>SKIVKIIGREIIDSRGNPTVEAEVHLEGGFVGMAAAPSGASTGSREALELRDGDKSRFLGKGVTKAVAAVNGPIAQALIGKDAKD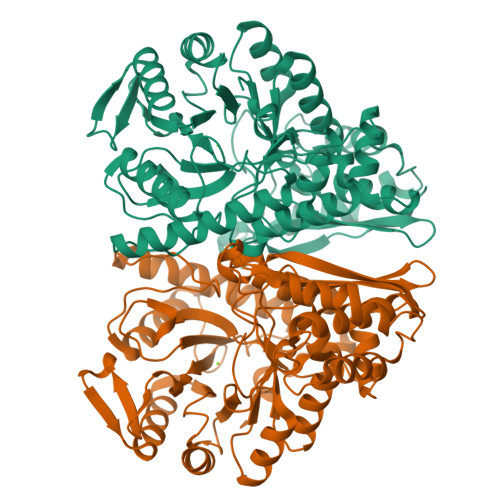QAGIDKIMIDLDGTENKSKFGANAILAVSLANAKAAAAAKGMPLYEHIAELNGTPGKYSMPVPMMNIINGGEHADNNVDIQEFMIQPVGAKTVKEAIRMGSEVFHHLAKVLKAKGMNTAVGDEGGYAPNLGSNAEALAVIAEAVKAAGYELGKDITLAMDCAASEFYKDGKYVLAGEGNKAFTSEEFTHFLEELTKQYPIVSIEDGLDESDWDGFAYQTKVLGDKIQLVGDDLFVTNTKILKEGIEKGIANSILIKFNQIGSLTETLAAIKMAKDAGYTAVISHRSGETEDATIADLAVGTAAGQIKTGSMSRSDRVAKYNQLIRIEEALGEKAPYNGRKEIKGQA[4x]> MNINDNLSINSPVDNKNVVVVRARKTDTVFKAFKVAPNIWVAPERYYGESLSIDEEYKVDGGIYDSNFLSQDSEKDKFLQAIITLLKRINSTNAGEKLLSLISTAIPFPYGYIGGGYYAPNMITFGSAPKSNKKLNSLISSTIPFPYAGYRETNYLSSEDNKSFYASNIVIFGPGANIVENNTVFYKKEDAENGMGTMTEIWFQPFLTYKYDEFYIDPAIELIKCLIKSLYFLYGIKPSDDLVIPYRLRSELENIEYSQLNIVDLLVSGGIDPKFINTDPYWFTDNYFSNAKKVFEDHRNIYETQIEGNNAIGNDIKLRLKQKFRININDIWELNLNYFSKEFSIMMPDRFNNALKHFYRKQYYKIDYPENYSINGFVNGQINVQLSLSDRNQDIINKPEEIINLLNGNNVSLMRSNIYGDGLKSTVDDFYSNYKIPYNRAYEYHFNNSNDSSLDNVNIGVIDNIPEIIDVNPYKENCDKFSPVQKITSTREINTNIPWPINYLQAQNTNNEKFSLSSDFVEVVSSKDKSLVYSFLSNVMFYLDSIKDNSPIDTDKKYYLWLREIFRNYSFDITATQEINTDCGINKVVTWFGKALNILNTSDSFVEEFQNLGPISLINKKENLSMPIIEIYGIPNDMLGLPLNDLNEKLFNIYLKNILYFKKVYFNFLDQWWTEYYSQYFDLICMAKQSILAQEKLIKQIIQNKLQDLFKADISMDKLNLMNLATEKTFIDLSNESQIAINNINDFLNKSAICVFDTNIYPKFISFMEQCINSVNSNVTAFIQKCTNITEDEKLQLIKLNTFMNIDFEFFDIQSIKDLITSETDLIKEEKESDYNLFLFTLQEDNNKVIEDISGKNTLVKYSDSISLVYGVNGDALYLKEPDESVSFSNKAFENGLTNSFSICFWLRNLGEDIITSKLIENKADNCGWEIYFENNGLVFSIVDCNGNEENIYLSDVISKNWYYISISIDRLRNQLLIFINDKLIANQSIEQILNIYSSNTISLVNENNPIYIEGLSILNRSITSEEVVNNYFSYLNNSYIRDISGERLEYNKTYELYNYVFPENSLYEVTENNNIYLSI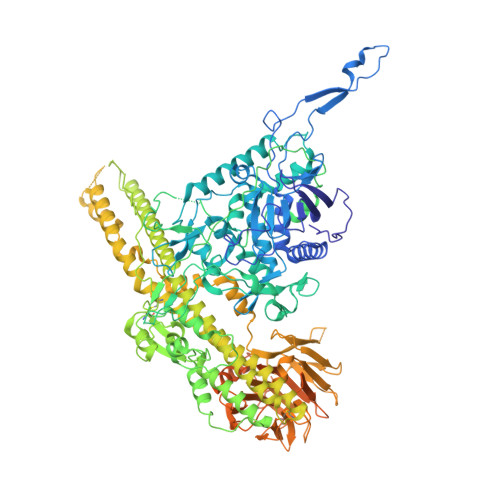KDTNNLNIQGAKFKLINIDANKQYVQKWDEGVVCLLGDEEKYVDISSENNRIQLVNSKDTAKRIIFNNDIFMPNCLTFAYNNKYLSLSLRDRNYNWMICNNNDNIPKAAHLWALKGI>[2x]MGLEEKKENKQLTYTTVKDIGDMNPHVYGGSMSAESMIYEPLVRNTKDGIKPLLAKKWDVSEDGKTYTFHLRDDVKFHDGTPFDADAVKKNIDAVQENKKLHSWLKISTLIDNVKVKDKYTVELNL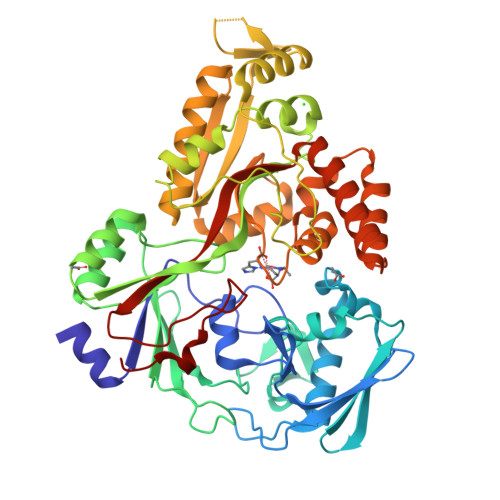KEAYQPALAELAMPRPYVFVSPKDFKNGTTKDGVKKFDGTGPFKLGEHKKDESADFNKNDQYWGEKSKLNKVQAKVMPAGETAFLSMKKGETNFAFTDDRGTDSLDKDSLKQLKDTGDYQVKRSQPMNTKMLVVNSGKKDNAVSDKTVRQAIGHMVNRDKIAKEILDGQEKPATQLFAKNVTDINFDMPTRKYDLKKAESLLDEAGWKKGKDSDVRQKDGKNLEMAMYYDKGSSSQKEQAEYLQAEFKKMGIKLNINGETSDKIAERRTSGDYDLMFNQTWGLLYDPQSTIAAFKAKNGYESATSGIENKDKIYNSIDDAFKIQNGKERSDAYKNILKQIDDEGIFIPISHGSMTVVAPKDLEKVSFTQSQYELPFNEMQYK> VLIPSHAQRDLT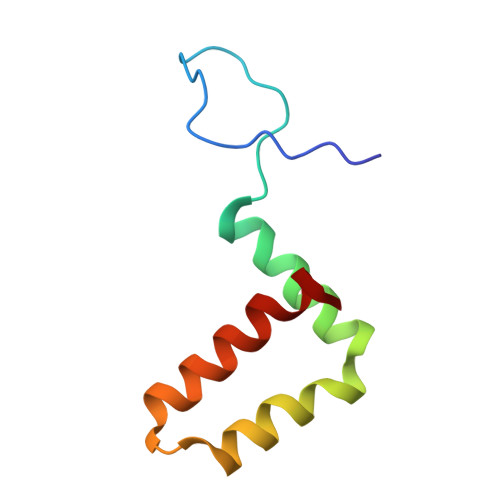GRGHQWLEGEAVKAHLTRVEGWVWKNKLFTLSLVMVAWLMVDGLLPRILIVVVALALAPAYA> PHMGLEEKKENKQLTYTTVKDIGDMNPHVYGGSMSAESMIYEPLVRNTKDGIKPLLAKKWDVSEDGKTYTFHLRDDVKFHDGTPFDADAVKKNIDAVQENKKLHSWLKISTLIDNVKVKDKYTVELNLKEAYQPALAELAMPRPYVFVSPKDFKNGTTKDGVKKFDGTGPFKLG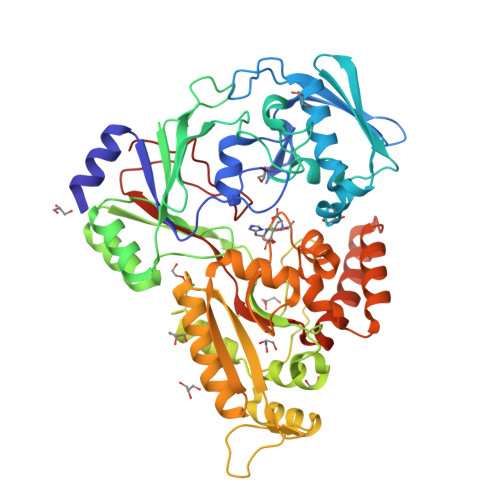EHKKDESADFNKNDQYWGEKSKLNKVQAKVMPAGETAFLSMKKGETNFAFTDDRGTDSLDKDSLKQLKDTGDYQVKRSQPMNTKMLVVNSGKKDNAVSDKTVRQAIGHMVNRDKIAKEILDGQEKPATQLFAKNVTDINFDMPTRKYDLKKAESLLDEAGWKKGKDSDVRQKDGKNLEMAMYYDKGSSSQKEQAEYLQAEFKKMGIKLNINGETSDKIAERRTSGDYDLMFNQTWGLLYDPQSTIAAFKAKNGYESATSGIENKDKIYNSIDDAFKIQNGKERSDAYKNILKQIDDEGIFIPISHGSMTVVAPKDLEKVSFTQSQYELPFNEMQYK>FKFEFKFE[1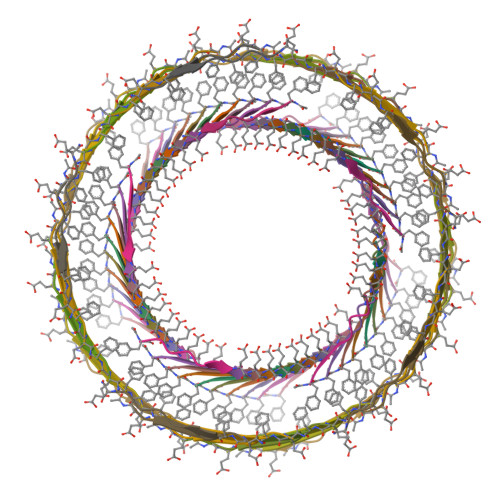00x]>[10x]YKDDDDKLHSQANLMRLKSDLFNRSPMYPGPTKDDPLTVTLGFTLQDIVKADSSTNEVDLVYYEQQRWKLN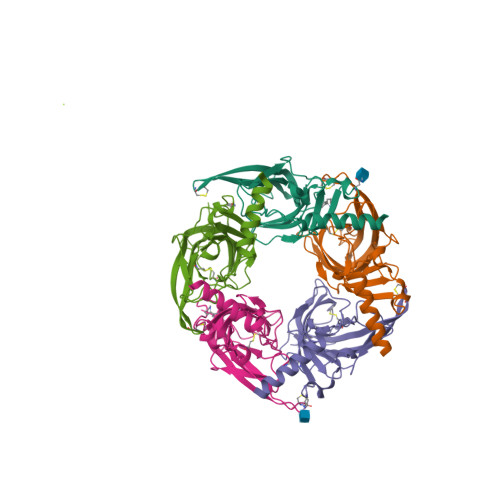SLMWDPNEYGNITDFRTSAADIWTPDITAYSSTRPVQVLSPQIAVVTHDGSVMFIPAQRLSFMCDPTGVDSEEGATCAVKFGSWVYSGFEIDLKTDTDQVDLSSYYASSKYEILSATQTRQVQHYSCCPEPYIDVNLVVKFRERRAGNGFFRNLFD>[2x]KSCCRSTLGRNCYNLCRVRGAQKL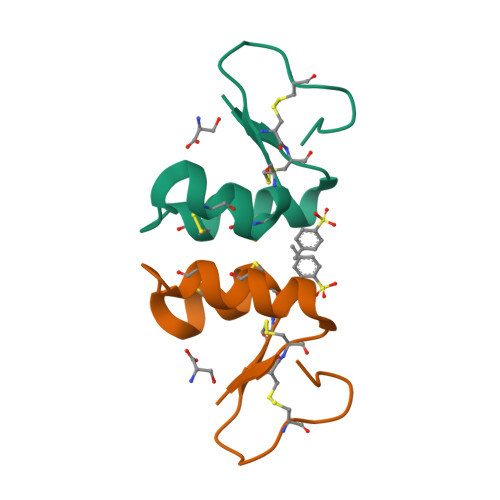CANACRCKLTSGLKCPSSFPK>[4x]MHSRFQAALTTLAADLQAAIAPMLADPHFPALLEADQVATLQHATGLDEDALAFALLPLAAACARPDLSHFNVGAIARGVSGRWYFGGNMEFLGATMQQTVHAEQSAISHAWLRGETSLRAITVNYTPCGHCRQFMNELNSGLALRIHLPGREAHALEHYLPDAFGPKDLEIKTLLMDEQ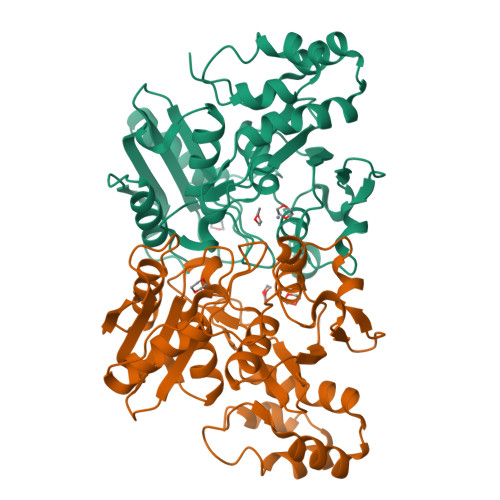DHGFPVSGDALTQAAIQAANRCHAPYSHSPSGVALELKDGTIFSGSYAENAAFNPTLPPLQGALNLLSLNGYDYPAIQRAILAEKADAALIQWDATVATLKALGCHNIERVLLG> 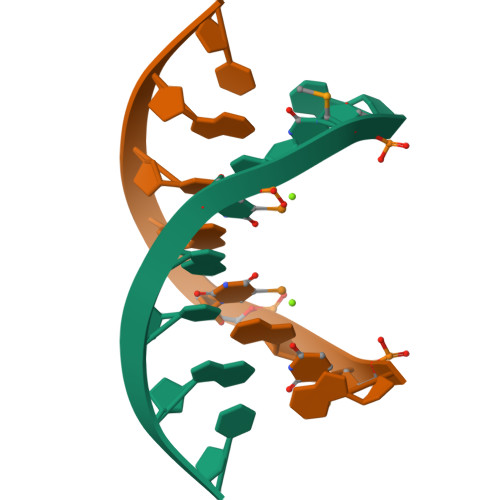GUGUACAC> MHHHHHHSSGRENLYFQGKERRRAVLELLQRPGNARCADCGAPDPDWASYTLGVFICLSCSGIHRNIPQVSKVKSVRLDAWEEAQVEF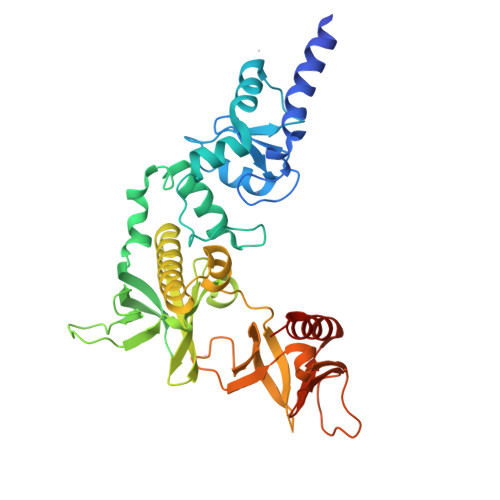MASHGNDAARARFESKVPSFYYRPTPSDCQLLREQWIRAKYERQEFIYPEKQEPYSAGYREGFLWKRGRDNGQFLSRKFVLTEREGALKYFNRNDAKEPKAVMKIEHLNATFQPAKIGHPHGLQVTYLKDNSTRNIFIYHEDGKEIVDWFNALRAARFHYLQVAFPGASDADLVPKLSRNYLKEGYMEKTGPKQTEGFRKRWFTMDDRRLMYFKDPLDAFARGEVFIGSKESGYTVLHGFPPSTQGHHWPHGITIVTPDRKFLFACETESDQREWVAAFQKAVDRPMLPQEYAVEAHF>ALALDTPLPTPSGWTTMGDVAVGDHLLGPDGEPTR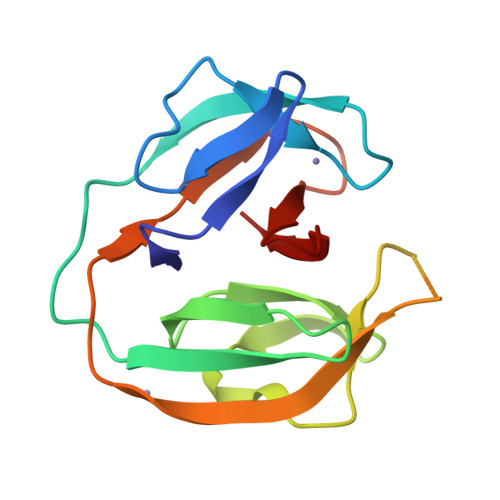VVADTDVMLGRPCYVVEFSDGTAIVADAQHQWPTEHGVRITANLRAGMHTVVSASGGRGGTALLAPAVQITAVRRRPSVPVRCVEVDNPEHLYLAGPGMVPTHN[3x]>[4x]MKQQAIDEQLRNAIEYTPEMFTQVPMLYINIEINNYPVKAFVDTGAQTTIMSTRLAKKTGLSRMIDKRFIGEARGVGTGKIIGRIHQAQVKIETQYIPCS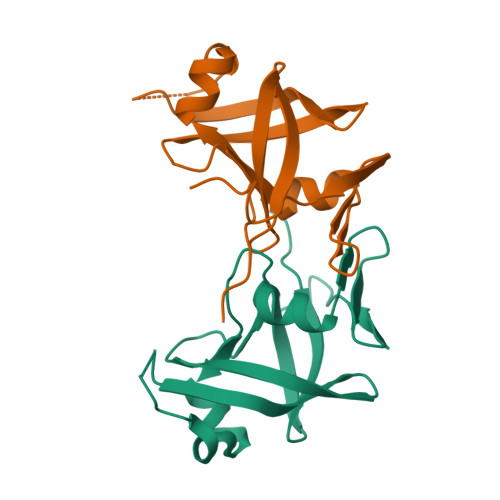FTVLDTDIDVLIGLDMLKRHLACVDLKENVLRIAEVETSFLSEAEIPK> MGIKVTKDLVLHLENLARLELSEDQRESLMKDFQEILDYVE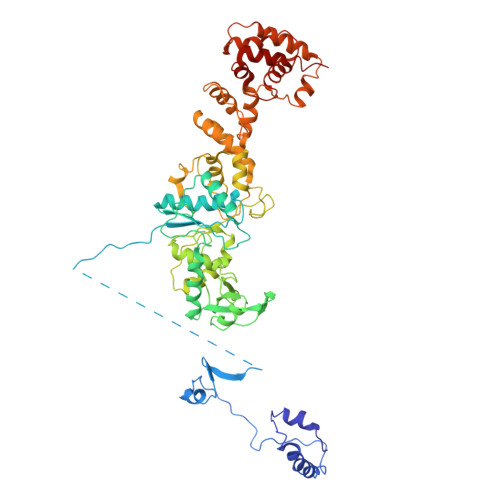LLNEVDVEGVEPMYTPVEDSAKLRKGDPRFFEMRDLIKKNFPEEKDGHIKVPGIHRGSGSGSGSMFITGAFFDILEVGPKKIRRCFELVRVRFAPSPTGHLHVGGARTALFNWMFARKEGGKFILRIEDTDTERSSREYEQQILESLRWCGLDWDEGPDIGGDFGPYRQSERLEIYREYAEKLVEDKRAYYVVYDKEDPSKELFTTYEYPHEYKEKGHPVTIKFKVLPGKTSFEDLLKGYMEFDNSTLEDFIIMKSNGFPTYNFAVVVDDHLMRISHVFRGEDHLSNTPKQLMIYEAFGWEAPVFMHIPLILGSDRTPLSKRHGATSVEHFRREGILSRALMNYLALLGWRVEGDEIFTIEEKLQSFDPKDISNKGVIFDYQKLEWVNGKHMRRIDLEDLKREFIEWAKYAGKEIPSVDERYFSETLRICREKVNTLSQLYDIMYPFMNDDYEYEKDYVEKFLKREEAERVLEEAKKAFKDLNSWNMEEIEKTLRDLSEKGLASKKVVFQLIRGAVTGKLVTPGLFETIEVLGKERTLKRLERTLQFLKKT> AYTTFSQTKNDQLKEPMFFGQPVNVARYDQQKYD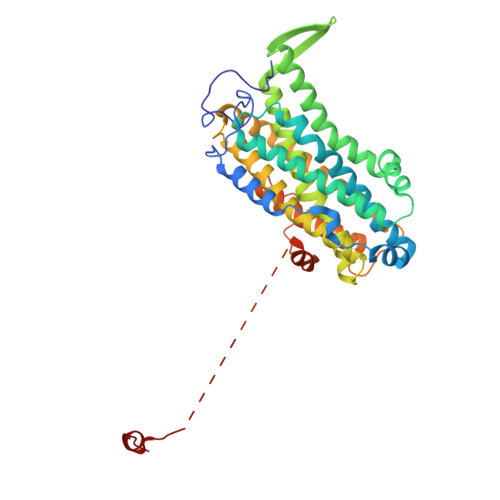IFEKLIEKQLSFFWRPEEVDVSRDRIDYQALPEHEKHIFISNLKYQTLLDSIQGRSPNVALLPLISIPELETWVETWAFSETIHSRSYTHIIRNIVNDPSVVFDDIVTNEQIQKRAEGISSYYDELIEMTSYWHLLGEGTHTVNGKTVTVSLRELKKKLYLCLMSVNALEAIRFYVSFACSFAFAERELMEGNAKIIRLIARDEALHLTGTQHMLNLLRSGADDPEMAEIAEECKQECYDLFVQAAQQEKDWADYLFRDGSMIGLNKDILCQYVEYITNIRMQAVGLDLPFQTRSNPIPWINTWLVSDNVQVAPQEVEVSSYLVGQIDSEVDTDDLSNFQL~{N}1,~{N}1,~{N}8,~{N}8-tetramethylnaphthalene-1,8-diamine | C14 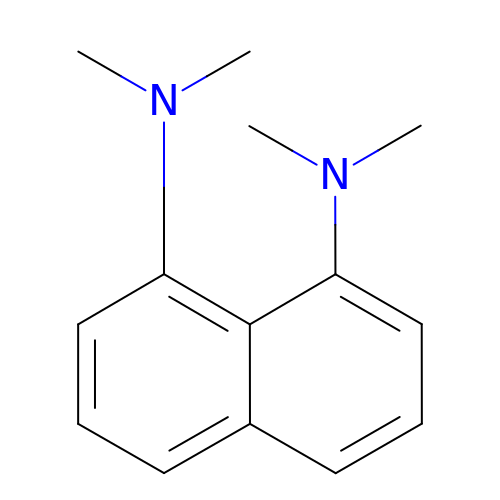H18 N2 | GJFNRSDCSTVPCJ-UHFFFAOYSA-N> GPGSLTVGDWLDSIRMGRYRDHFAAGGYSSLGMVLRMNAQDVRALGITLMGHQKKILGSIQT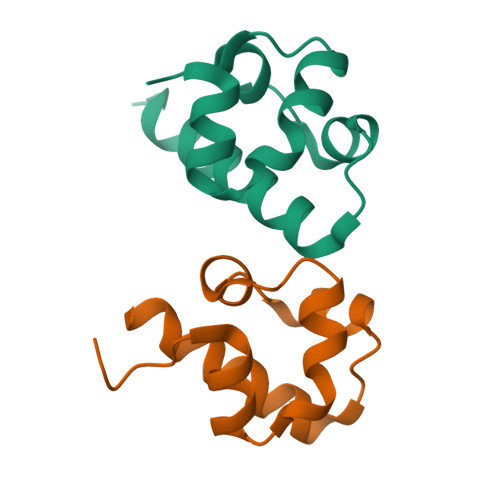MRAQLSS;> GPGSEFPSQPKSVEDLLDRINLKEHMPTFLFNGYEDLDTFKLLEEEDLDELNIRDPEHRAVLLTAVELLQEYD>MRPPQFTRAQWFAIQHISLNPPRCTIAMRAINNYRWRCKNQNTFLRTTFANVVNVCGNQSIRCPHNRTLNNCHRSRFRVPLLHCDLINPGAQ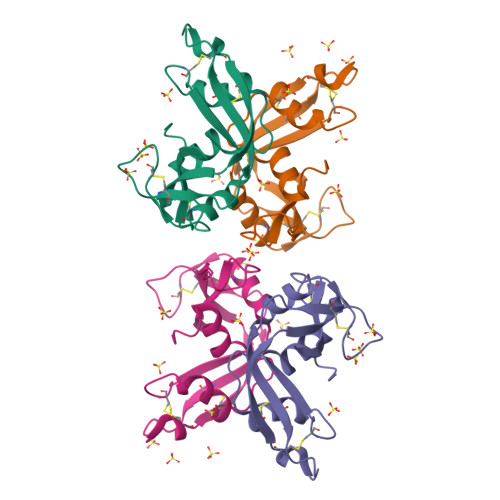NISNCRYADRPGRRFYVVACDNRDPRDSPRYPVVPVHLDTTI[2x]> AHAFWST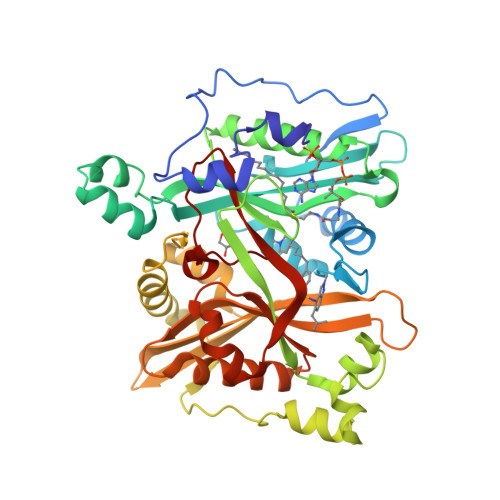QPVPQTEDETEKIVFAGPMDEPKTVADIPEEPYPIASTFEWWTPNMEAADDIHAIYELLRDNYVEDDDSMFRFNYSEEFLQWALCPPNYIPDWHVAVRRKADKKLLAFIAGVPVTLRMGTPKYMKVKAQEKGEGEEAAKYDEPRHICEINFLCVHKQLREKRLAPILIKEATRRVNRTNVWQAVYTAGVLLPTPYASGQYFHRSLNPEKLVEIRFAGAPAQYAAFANPMAMLKRNYQLPSAPKNSGLREMKPSDVPQVRRILMNYLDSFDVGPVFSDAEISHYLLPRDGVVFTYVVENDKKVTDFFSFYRIPSTVIGNANYNLLNAAYVHYYAATSIPLHQLILDLLIVAHSRGFDVCNMVEILDNRSFVEQLKFGAGDGHLRYYFYNWAYPKIKPSQVALVML> MDKKSLYKYLLLRSTGDMHRAKSPTIMTRVTNNVYLGNYKNAMDAPSSEVKFKYVLNLTMDKYTLPNSNINIIHIPLVDDTTTDISKYFDDVTAFLSKCDQRNEPVLVHCVAGVNRSGAMILAYLMSKNKESSPMLYFLYVYHSMRDLRGAFVENPSFKRQIIEKYVIDKN

Poxviruses express a dual specific phosphatase (H1) that de-phosphorylates signal transducer and activator of transcription 1 (STAT1) and blocks interferon signal transduction. H1 is conserved in poxviruses and is essential for virus replication in cell culture. Due to the importance of H1 in modulating interferon-signaling and viral replication, it serves as an attractive anti-poxvirus drug target.

To understand the mechanism for monkeypox H1 catalyzed dephosphorylation and provide an accurate structural model for drug discovery, we determined a crystal structure of H1 to 1.8 Å resolution. Monkeypox H1 has 171 amino acid residues and the refined model includes residues 2–171 with well-fitting electron density. Two H1 molecules are related by crystallographic symmetry and form a domain swapped dimer, which resembles a butterfly. The overall structure is composed of six α helices and four β strands. The N-terminal helix α1 from each protomer interchanges to mediate H1 dimerization. Size exclusion chromatography confirms the H1 dimer in solution, suggesting that dimerization represents its functional state. The H1 active site consists of a Cys-Arg-Asp catalytic triad. The arginine residue (Arg116) of this loop captures the phosphate ion, whose guanidinium group interacts with two phosphate oxygens through two hydrogen bonds with the distances of 2.9 and 3.0 Å, respectively. There is a phosphate ion captured at each active site, representing the final stage of catalysis before the product is released. The first hot spot is the dimer interface, which is unique among the members in the protein tyrosine phosphatase (PTP)/dual-specificity phosphatase (DSP) family.In eukaryotes, wobble uridines are modified by Elongator, a large and highly conserved macromolecular complex. Elongator consists of two subcomplexes, namely Elp123 containing the enzymatically active Elp3 subunit and the associated Elp456 hetero-hexamer. The Elongator complex harbors two copies of each of its six subunits, namely Elongator proteins 1–6 (Elp1–Elp6). Decreased levels of wobble uridine modifications lead to ribosome pausing, incorrect protein folding and consequently trigger intracellular protein aggregation and proteotoxic stress.

To determine the structure of MmElp123, we vitrified freshly purified samples in absence and presence of in vitro transcribed mouse tRNA ArgUCU. We optimized the sample preparation procedure, collected large datasets and solved structures that are with and without tRNA at 4.35 Å and 4.0 Å resolutions, respectively. As for the mouse apo Elp123 structure, the obtained density is significantly smaller and only the core lobe of the subcomplex is structured, resulting in decreased overall dimensions (∼140 × 100 × 65 Å). In detail, the spatial arrangement of Elp2, Elp3 and the N-terminal region of Elp1 are very similar to the tRNA-bound MmElp123 and the ScElp123 structures. Strikingly, the CTD of MmElp1, which is visible in the yeast Elp123, remains flexible in MmElp123 in the absence of tRNA. This observation indicates that yeast Elp123 is inherently more stable in the absence of tRNAs and that the binding of tRNAs induces structural rearrangements in the Elp1 CTD of mammals. Surprisingly, we could identify an intact SAM molecule bound to the iron-sulfur cluster of MmElp123, which was co-purified from the host cells. The coordination of this ligand is similar to the 5′-dA molecule found in ScElp123. Nonetheless, the structural similarities between the subcomplexes (pre and post SAM cleavage), suggest that the cleavage reaction itself does not induce major rearrangements in the active site of Elp3 or in the coordination of the adenosine moiety. First, the MmElp123 harbors a SAM molecule that is bound to the iron-sulfur cluster, indicating that SAM binding occurs before tRNA binding.

> MRNLKLHRTLEFRDIQAPGKPQCFCLRAEQGTVLIGSERGLTEVDPVRREVKTEISLVAEGFLPEDGSGCIVGIQDLLDQESVCVATASGDVIVCNLSTQQLECVGSVASGISVMSWSPDQELLLLATAQQTLIMMTKDFEVIAEEQIHQDDFGEGKFVTVGWGSKQTQFHGSEGRPTAFPVQLPENALPWDDRRPHITWRGDGQYFAVSVVCRQTEARKIRVWNREFALQSTSESVPGLGPALAWKPSGSLIASTQDKPNQQDVVFFEKNGLLHGHFTLPFLKDEVKVNDLLWNADSSVLAIWLEDLPKEDSSTLKSYVQLWTVGNYHWYLKQSLPFSTTGKNQIVSLLWDPVTPCRLHVLCTGWRYLCCDWHWTTDRSSGNSANDLANVAVIDGNRVLVTVFRQTVVPPPMCTYRLLIPHPVNQVIFSAHLGNDLAVLDASNQISVYKCGDKPNMDSTVKLGAVGGNGFKVPLTTPHLEKRYSIQFGNNEEEEEEEVNALQLSFLTWVEDDTFLAISYSHSSSQSIIHHLTVTHSEVDEEQGQLDVSSSVTVDGVVIGLCCCSKTKSLAVQLADGQVLKYLWESPSLAVEPWKNSEGIPVRFVHPCTQMEVATIGGEECVLGLTDRCRFFINDTEVASNITSFAVCDDFLLVTTHSHTCQVFSLSGASLKMLQAALSGSHEASGEILRKVERGSRIVTVVPQDTKLILQMPRGNLEVVHHRALVLAQIRKWLDKLMFKEAFECMRKLRINLNLIHDHNPKVFLENVETFVKQIDSVNHINLFFTELREEDVTKTMYPPPITKSVQVSTHPDGKKLDLICDAMRAAMEAINPRKFCLSILTSHVKKTTPELEIVLQKVQELQGNLPFDPESVSVEEALKYLLLLVDVNELFNHSLGTYDFNLVLMVAEKSQKDPKEYLPFLNTLKKMETNYQRFTIDKYLKRYEKALGHLSKCGPEYFTECLNLIKDKNLYKEALKLYRPDSPQYQAVSMAYGEHLMQEHLYEPAGLVFARCGAQEKALEAFLACGSWQQALCVAAQLQMSKDKVAGLARTLAGKLVEQRKHSEAATVLEQYAQDYEEAVLLLLEGSAWEEALRLVYKYDRVDIIETSVKPSILEAQKNYMDFLDSETATFIRHKNRLQVVRALRRQAPQVHVDHEVAHGPESDLFSETSSIMSGSEMSGRYSHSNSRISARSSKNRRKAERKKHSLKEGSPLEGLALLEALSEVVQSVEKLKDEVRAILKVLFLFEFEEQAKELQRAFESTLQLMERAVPEIWTPAGQQSSTTPVLGPSSTANSITASYQQQKTCVPALDAGVYMPPKMDPRSQWKLSLLE;> MVSSVLEVSHVFCCPNRVRGALSWNTGPGGLLAFGTSCSVVLYDPQKKVVITNLNGHTARVNCLQWIRTEDGSPSNELVSGGSDNRVIHWELENNQVLKSVRLQGHEGPVCAVHAIYQSGPSEGEQHALIASAASDSTVRIWSKKGSEVKYLQTLSFRDGFVLSVCLAILPGTNVPVLACGDDDCRIHLYIQQDDQFQKALSLCGHEDWIRGVEWATFGRDLFLASCSQDCLIRIWRLYMKPASFETKDGSLRLKENTFTIKDGGVRTTVAVTLETVLAGHENWVNAVHWQPSFYKDGVLQQPVRLLSASMDKTMILWAPDEESGVWLEQVRVGEVGGNTLGFYDCQFGENGTMIIAHAFHGALHLWKQSTVNPRQWAPEIVISGHFDGVQDLMWDPEGEFIITTSTDQTTRLFAPWKKKDQKDRSQVTWHEIARPQIHGYNIKCLAMIDRFQFVSGADEKVLRVFSAPRNFVENFSVISRQSLSHMLCDDQDLPEGATVPALGLSNKALFQGDIASQPFEEDELISPAFGSPQVTFQPAVLNEPPTEDHLLQNTLWPEIQKLYGHGYEIVCVACNNSKTLLASACKASQKEHAAIILWSTASWKQVQSLAFHTLTVTQMTFSPDDKFLLAVSRDRTWSLWKRQDATSSEFDPFFSLFAFTNKITSVHSRIIWSCDWSPDNKYFFTGSRDKKVVVWGECKSSHNPMEHPIRPCSSILDVGSSVTAVSVCPVLNPAQRYIVAIGLESGKICIYSWNKTNQEINDWTSCVETNPSQSHSLGIRRLCWKSCSDDDDDDDDDDTEQSEEGPEWLHFASCGEDHTVKIYRVNRRAL;> MRQKRKGDLSPAELMMLTIGDVIKQLVEAHEQGKDVDLNKMKTKTAAKYGLASQPRLVDIIAAVPPHYRKILIPKLKAKPVRTASGIAVVAVMCKPHRCPHISFTGNICIYCPGGPDSDFEYSTQSYTGYEPTSMRAIRARYDPFLQTRHRIEQLKQLGHSVDKVEFIVMGGTFMALPEEYRDYFIRSLHDALSGHTSNNIHEAIKYSERSFTKCVGITIETRPDYCMKRHLSDMLTYGCTRLEIGVQSVYEDVARDTNRGHTVKAACESFHLAKDSGFKVVTHMMPDLPNVGLERDIEQFIEFFENPAFRPDGLKLYPTLVIRGTGLYELWKSGRYRSYSPSDLIELVARILALVPPWTRVYRVQRDIPMPLVSSGVEHGNLRELAFARMKDLGIQCRDVRTREVGIQEIHHRVRPYQVELVRRDYVANGGWETFLSYEDPDQDILIGLLRLRKCSEETFRFELGGGVSIVRELHVYGSVVPVSSRDPTKFQHQGFGMLLMEEAERIAREEHGSGKMAVISGVGTRNYYRKIGYRLQGPYMVKMLK(3S)-2-{(2R)-2-(cyclopentylmethyl)-3-[formyl(hydroxy)amino]propanoyl}-N-(pyridin-2-yl)hexahydropyridazine-3-carboxamide 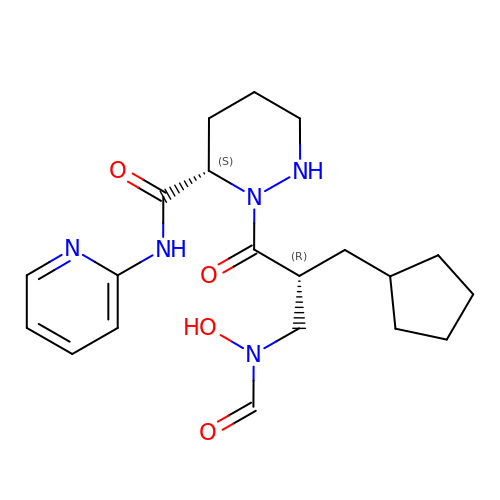| C20 H29 N5 O4 | IGYIJLMSSQSKHF-SJORKVTESA-N2-chloro-10-[3-(4-methylpiperazin-1-yl)propyl]-10H-phenothiazine | C20 H24 Cl N3 S | 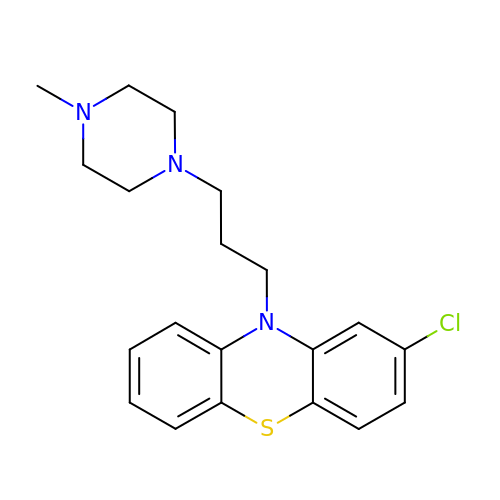WIKYUJGCLQQFNW-UHFFFAOYSA-N> KVFERCELARTLKRLGMDG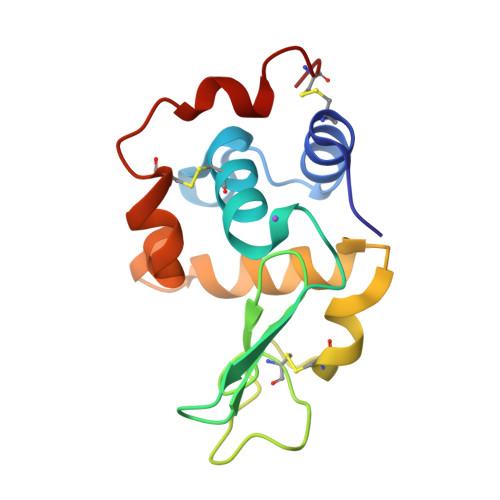YRGISLANWMCLAKWESGYNTRATNYNAGDRSTDYGIFQANSRYWCNDGKTPGAVNAAHLSCSALLQDNIADAVAAAKRVVRDPQGIRAWVAWRNRCQNRDVRQYVQGCGV> MKPKKRQMEYLTRGLIAVQ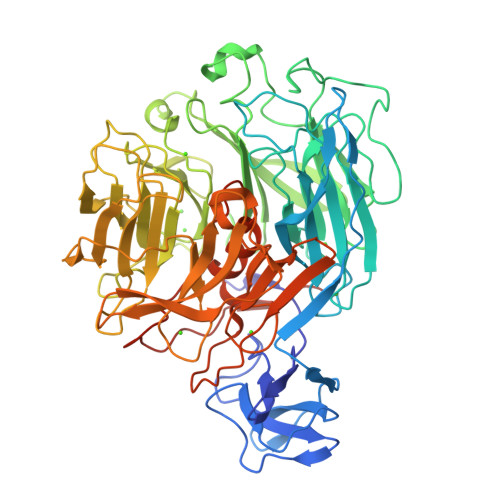TEQGVFVSWRFLGTDHETTAFHLYRDGKRITRDPIAESTNFLDQNGTADSVYQVAAVNKGREEKLSKKARVWQENVLEVPLAKPEGGVTPDGKPYTYSANDASVGDIDGDGEYEMILKWDPSNSKDNAHDGYTGEVLIDAYKLDGTFLWRINLGRNIRAGAHYTQFMVYDLDGDGKAEIAMKTADGTTDGKGHIIGDEQADFRNEQGRILSGPEYLTVFKGETGEALTTVEYEPPRGKLEDWGDGYGNRMDRFLAGTAYLDGERPSLVMARGYYTRTVLVAYDFRNGRLKKRWVFDSNQPGHEAYAGQGNHSLSVADVDGDGKDEIIYGAMAVDHDGTGLYSTGLGHGDAMHVGDLDPSRKGLEVFQVHEDATKPYGLSLRDAGTGEILWGVHAGTDVGRGMAAHIDPSYKGSLVWGIDPPGNDGMSYGLFTSKGEKISDKAPSSANFAIWWDGDLVRELLDHDWDGTIGRPKIEKWDAENGCLKTIFQPAGVLSNNGTKGNPVLQANLFGDWREEVIWRTEDSSALRIYTTTHLTRHCFYTLMHDPVYRLGIAWQNTAYNQPPHTSFYLGTGMKKPPKPALYIAGSKAEAPLLEHHHHHH The UNC-45 chaperone controls myosin function mediating the folding, assembly, and degradation of the muscle protein. UNC-45, which is present in all eukaryotes, employs a UCS domain to interact with myosin, a central domain that mediates oligomerization, and a TPR domain that interacts with members of the protein quality control (PQC) network. In addition to functioning as a folding factor of the myosin motor, UNC-45 can form linear protein chains that provide regular spaced docking sites for HSP70 and HSP90. Structural analysis of a minimal chaperone:substrate complex reveals that UNC-45 binds to a conserved FX3HY motif in the myosin motor domain.

Given the difficulties in obtaining a co-crystal structure with C. elegans UNC-45, we moved to the less complex fungal orthologue SHE4. Despite lacking the TPR-domain, SHE4 contains a functional UCS-domain for myosin binding.

> MNKVWDRIVGSDSADAQSVLKERCSSPKDVTDLLHVIQNWTSEIHNNGEETRCWKCVPMLAGYVKDWGQLEFLCRRILLRSSIQEIRPLLLVTMKSLMSNHSDNTEQKCGNILQQLLIEAEEDSGNVSLRLLVDAMSLVFPICLGVCRDMFLSTDFQDILTRNLNSSADDEHLVNGALRLLAVSCIDEAVRRFIAEHYLKTLQQSFKVEKYKVLTALVLIKIWSFTKIEKETLNSCINLFIDSLSNGENIEINTEALAYLTLKPSVRVLLRGNGDVCLKIIELIKSQDTTPTDLYGLLIILANVSEHPSQNEDTVDKLKASLKTNQEKNDEPTLENVKDIEEFNRDYIIDLDLIGSLKSIKLSTSSYNQAIRIIYNVTRDKTQISECVKQGAGLMLLVFLAQKRNLSKDEWYLLSIRALSKTLIYVNPETAFSKYSPLSAAPFLFENLPLPNDNALSELQFTQLDTYEALLALTNLATINQGVDLGKIILSNAQYWDSIENLLLDSSVRIQRSTLELISNLMSNPMAISAKFFCFENPKSAQNFEILVKLLELHDIQSQRAVAAIFANIASTVPFICKELSEKRNLIETAIRVFKTQNTDTDLRIRLLVLLSSIFNANAHAVACVKNDEEFVKELQKYRNTPSQKDPLTPELSKEILSLINLEHHHHHH> MMRKSLCCALLLGISCSALATPVSEKQLAEVVANTITPLMKAQSVPGMAVAVIYQGKPHYYTFGKADIAANKPVTPQTLFELGSISKTFTGVLGGDAIARGEISLDDAVTRYWPQLTGKQWQGIRMLDLATYTAGGLPLQVPDEVTDNASLLRFYQNWQPQWKPGTTRLYANASIGLFGALAVKPSGMPYEQAMTTRVLKPLKLDHTWINVPKAEEAHYAWGYRDGKAVRVSPGMLDAQAYGV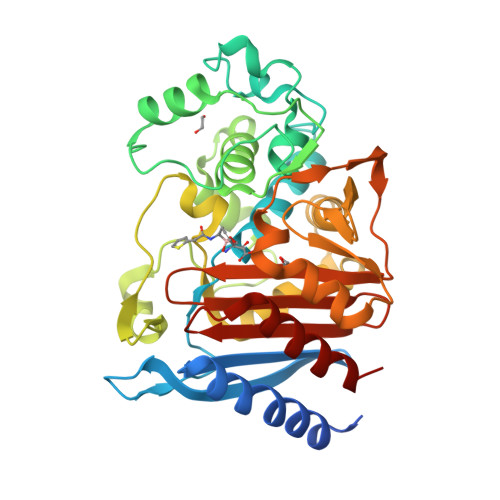KTNVQDMANWVMANMAPENVADASLKQGIALAQSRYWRIGSMYQGLGWEMLNWPVEANTVVEGSDSKVALAPLPVAEVNPPAPPVKASWVHKTGSTGGFGSYVAFIPEKQIGIVMLANTSYPNPARVEAAYHILEALQLE>GVDRDYLQ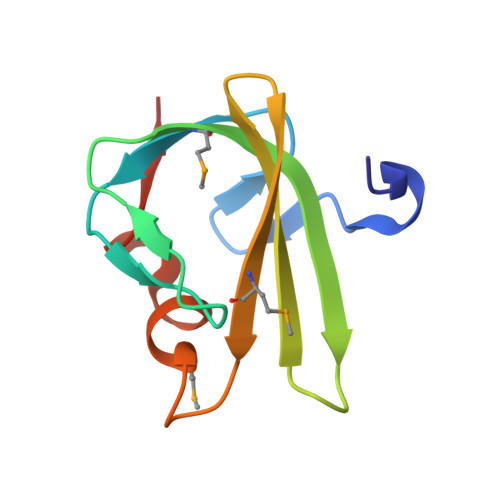SEYGVLKAGQCYKVVRSFRDYRNINYERGDVMRFLGSNFVPYESGLSLFFDKNGSERQIMLCVRPEFQMEIAHHLDSYFCKLDDN[2x]>[2x]SVQAD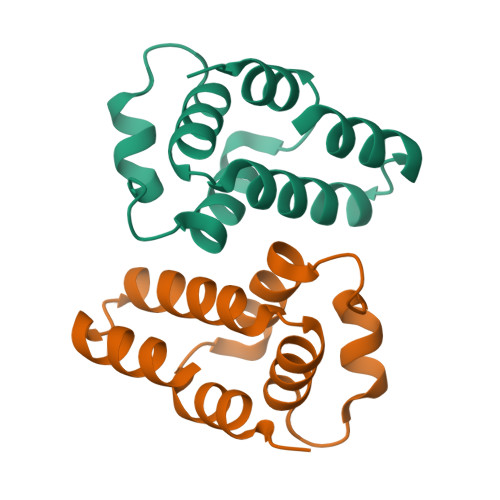YSRAEALAAWTRLSDEFIGNCYVSVRPRHAPAWEVVVASAAGSLRLEAFKRAHDHDFLDRLAVAIGNWEQKAQRPDHEIAQMLDQVG>GASQFFKDNCNRITASLVEGVELTKYISDINNNTDGMYVVSSTGGVWRISRAKDYPDNVMTAEMRKIAMAAVLSGMRVNMCASPASSPNVIWAIELEA[20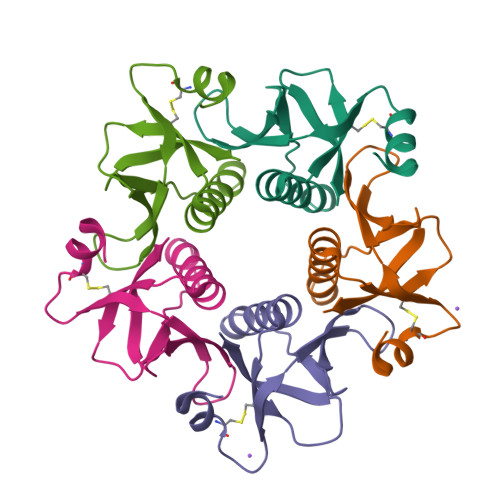x]>[4x]DPTIFEERHLKYISQLGKGNFGSVEL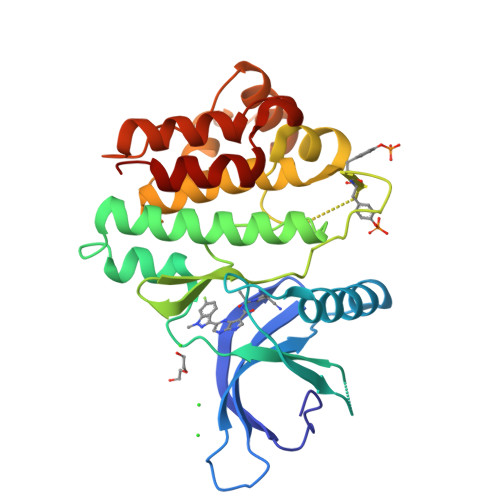CRYDPLGDNTGALVAVKQLQHSGPDQQRDFQREIQILKALHSDFIVKYRGVSYGPGRQSLRLVMEYLPSGCLRDFLQRHRARLDASRLLLYSSQICKGMEYLGSRRCVHRDLAARNILVESEAHVKIADFGLAKLLPLDKDYYVVREPGQSPIFWYAPESLSDNIFSRQSDVWSFGVVLYELFTYCDKSCSPSAEFLRMMGSERDVPALSRLLELLEEGQRLPAPPACPAEVHELMKLCWAPSPQDRPSFSALGPQLDMLWS4-chloranyl-1-[[2-methoxy-4-(trifluoromethyl)phenyl]methyl]pyrazolo[3,4-d]pyrimidin-6-amine | 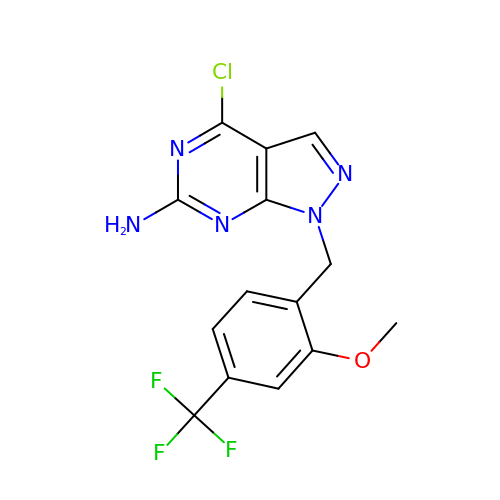C14 H11 Cl F3 N5 O | CRNFGOLKBZYMGM-UHFFFAOYSA-N>MGSSHHHHHHSSGLVPRGSHMTGAGLRWKHTSSLKVANEPVLAFTQGSPERDALQKALKDLKGRMEAIPCVVGDEEVWTSDVQYQVSPFNHGHKVAKFCYADKSLLNKAIEAALAARKEWDLKPIADRAQIFLKAADMLSGPRRAEILAKTMVGQGKTVIQAEIDAAAELIDFFRFNAKYAVELEGQQPISVPPSTNSTVYRGLEGFVAAISPFNFTAI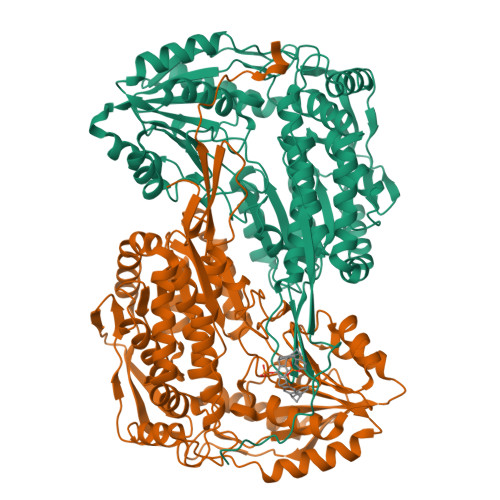GGNLAGAPALMGNVVLWKPSDTAMLASYAVYRILREAGLPPNIIQFVPADGPLFGDTVTSSEHLCGINFTGSVPTFKHLWKQVAQNLDRFHTFPRLAGECGGKNFHFVHRSADVESVVSGTLRSAFEYGGQKCSACSRLYVPHSLWPQIKGRLLEEHSRIKVGDPAEDFGTFFSAVIDAKSFARIKKWLEHARSSPSLTILAGGKCDDSVGYFVEPCIVESKDPQEPIMKEEIFGPVLSVYVYPDDKYKETLQLVDSTTSYGLTGAVFSQDKDVVQEATKVLRNAAGNFYINDKSTGSIVGQQPFGGARASGTNDKPGGPHYILRWTSPQVIKETHKPLGDWSYAYMQ[4x]(2R)-2-hydroxyhexanoic acid | C6 H12 O3 | 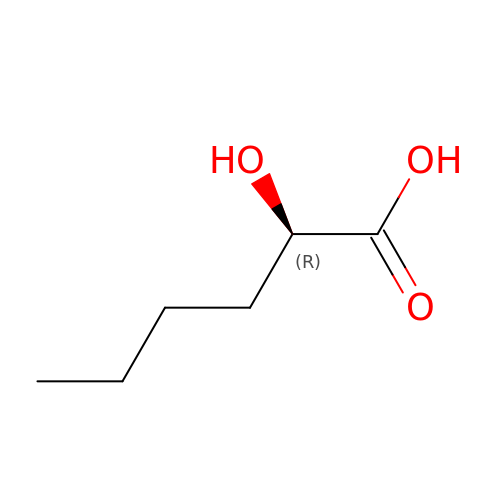NYHNVHGFPZAZGA-RXMQYKEDSA-N The DNA damage response protein 53BP1 (p53-binding protein 1) influences the cell cycle dependency of DNA double-strand break (DSB) repair pathway selection. The localization of 53BP1 to chromatin also requires that it binds histone H4 di-methylated at K20 (H4K20me2) via a tandem Tudor domain (53BP1TT), while BRCA1-BARD1 recruitment requires unmethylated H4K20 recognized by an Ankyrin repeat domain in BARD1. We show that a series of water-soluble small molecules targeting the methyl-lysine binding cavity in 53BP1TT function by stabilizing a previously unknown lowly populated autoinhibited homodimeric state of 53BP1TT in which the histone binding surface of H4K20me2 is buried within the protomeric interface. Our work therefore identifies an auto-associated form of 53BP1—autoinhibited for chromatin binding—that can be stabilized by small molecule ligands encapsulated between two 53BP1 protomers.

Our structural characterization of 53BP1TT in complex with the related compounds UNC2991 (Kd = 3.9 ± 0.4 μM), UNC3351 (Kd = 6.8 ± 0.4 μM) and UNC3474 (Kd = 1.0 ± 0.3 μM) revealed a similar three-dimensional (3D) arrangement wherein each ligand not only blocked the methyl-lysine binding site but was encapsulated in a cavity generated by two 53BP1TT molecules. This consistent burial of the histone binding surface of 53BP1TT by dimerization was unexpected. While crystallization could drive 53BP1TT homodimerization as has been shown for several other systems, that all four 3D structures were comparable despite differing crystallization conditions and space groups suggested that some 53BP1TT dimer may also exist in solution, even though all previous NMR spectroscopy studies only reported a monomeric state for 53BP1TT. Since the homodimerization interface in the crystal structures buries the histone binding surface of 53BP1TT, such a conformation would be autoinhibitory for chromatin binding. Titration of UNC2170, UNC2991, UNC3351 and UNC3474 into 15N-labeled 53BP1TT led to changes in several signal positions in the 1H−15N heteronuclear single quantum coherence (HSQC) NMR spectrum of 53BP1TT indicative of slow exchange on the chemical shift time scale. These chemical shift perturbations were more extensive than could be expected for just the small molecule binding surface and also mapped to amino acids located at the 53BP1TT dimer interface in our crystal structures. Several of the 53BP1TT residues that are close to the small molecule binding site had two different NMR signals. This is consistent with loss of symmetry observed in our crystal structures, allowing interactions by each of the two 53BP1TT protomers with a different “side” of the bound small molecule. Taken together, our data demonstrate that like in the crystal structures, the small molecules are buried at the interface of a 53BP1TT homodimer in solution.

>[10x]GHMNSFVGLRVVAKWSSNGYFYSGKITRDVGAGKYKLLFDDGYECDVLGKDILLCDPIPLDTEVTALSEDEYFSAGVVKGHRKESGELYYSIEKEGQRKWYKRMAVILSLEQGNRLREQYGLG>SMSDVTIVKEGWVQKRGEYIKNWRPRYFLLKTDGSFIGYKEKPQDVDLPYPLNNFSVAKCQLMKTERPKP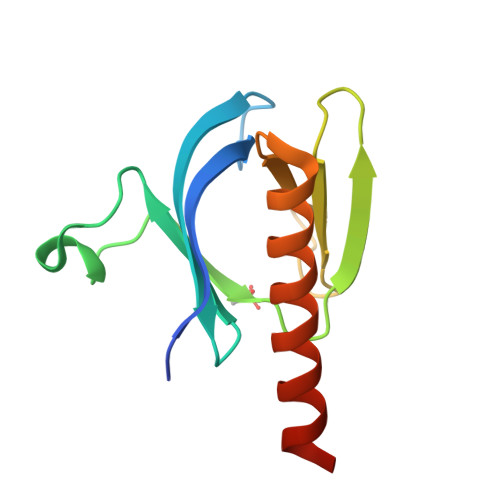NTFIIRCLQWTTVIERTFHVDTPEEREEWTEAIQAVADRLQRQEEERMN[8x]> QINQVRPKLPLLKILHAAGAQGEMFTVKEVMHYLGQYIMVKQ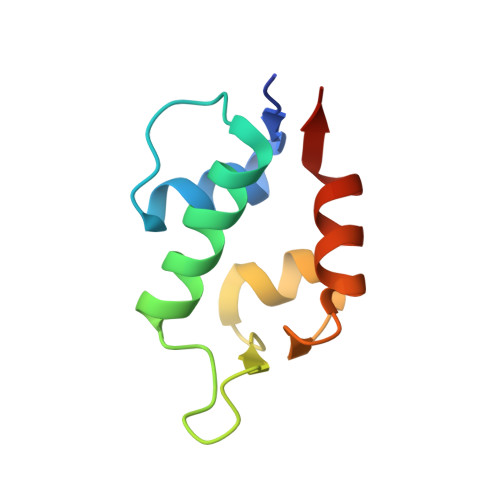LYDQQEQHMVYCGGDLLGELLGRQSFSVKDPSPLYDMLRKNLVTLAT>WSHPQFEKIEGRMSDGRESFLEVMRSVYERYLVGVPGVSEVWLIRHADSYTGLEDYDGDPRDPALSEKGRAQARLLAARLAGVPLHGVWASGAHRAQQTASAVAAEHGLRVRTDARLREVRTNWDDGRPSELKPHGVYPFPEPEKEVAERMRTAVTAAVAATPPAPDGTTRVAVVGHDSALVILMGSLMNLGWGQLDMILPLTSVSVLAVKDERMVVRSIGDA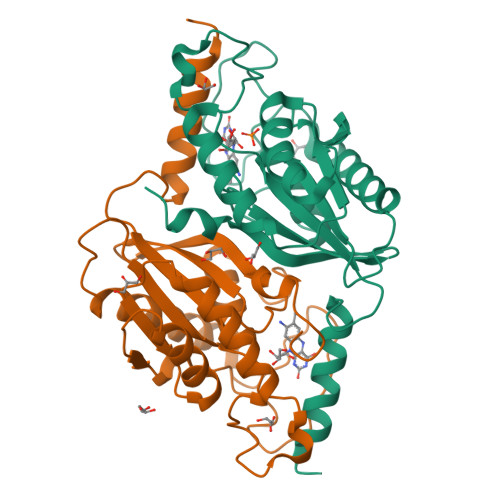THLAAAPSDVI[4x]>[2x]GUCUACCCACCUCGCC;>AGAGGA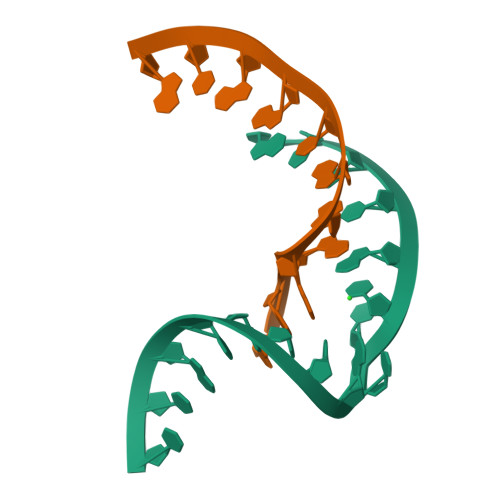CGGCG[2x]> GSH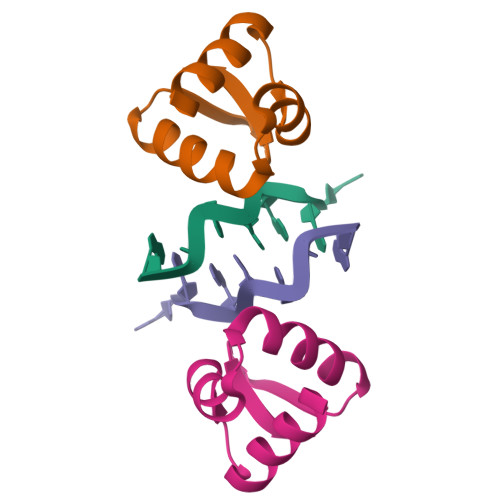MLSTGDNLEQKILQVLSDDGGPVKIGQLVKKCQVPKKTLNQVLYRLKKEDRVSSPEPATWSIGG> MEQRITLKDYAMRFGQTKTAKDLGVYQ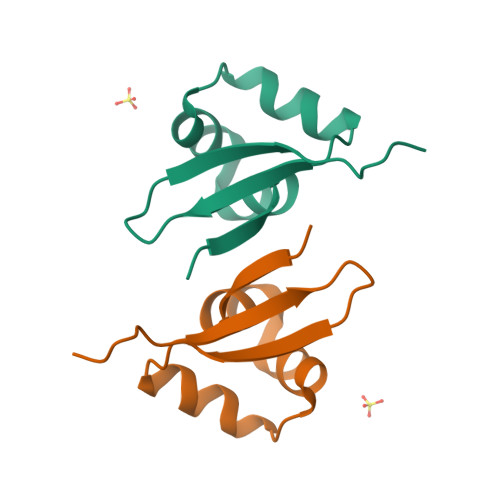SAINKAIHAGRKIFLTINADGSVYAEEVKPWPSN> MNDADVSKQIQ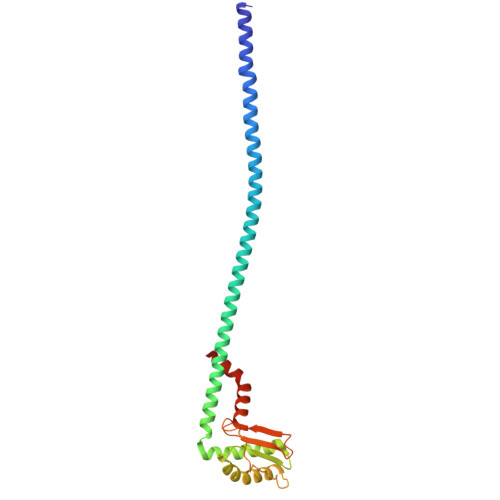QMVRFIRQEAEEKANEISVSAEEEFNIEKLQLVEAEKKKIRQEYERKEKQVEIRKKIEYSMQLNASRIKVLQAQDDLVSNMMEAASKEVLNVSRDHNSYKKLLKGLIVQSLLRLKEPAVLLRCRKDDHHLVESVLESAKEEYAQKLQVHPPEIIVDHHIYLPPGPGHHNAHGPSCSGGVVVASRDGKIVCENTLDARLDVVFRKKLPEIRKQLVSQVAA>SILKIHAREIFDSRGNPTVEVDLFTSKGLFRAAVPSGASTGIYEALELRDNDKTRYMGKGVSKAVEHINKTIAPALVSKKLNVTEQEKIDKLMIEMDGTENKSKFGANAILGVSLAVCKAGAVEKGVPLYRHIADLAGNSEVILPVPAFNVINGGSHAGNKLAMQEFMILPVGAANFREAMRIGAEVYHNLKNVIKEKYGKDATNVGDEGGFAPNILENKEGLELLKTAIGKAGYTDKVVIGMDVAASEFFRSGKYDLDFKSPDDPSRYISPDQLADLYKSFIKDYPVVSIEDPF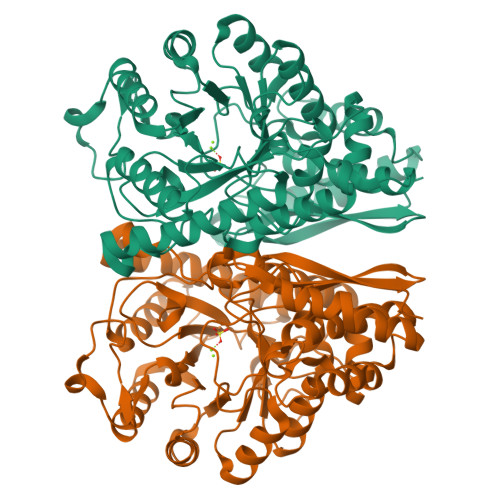DQDDWGAWQKFTASAGIQVVGDDLTVTNPKRIAKAVNEKSCNCLLLKVNQIGSVTESLQACKLAQANGWGVMVSHRSGETEDTFIADLVVGLCTGQIKTGAPCRSERLAKYNQLLRIEEELGSKAKFAGRNFRNPLAK[4x]4~{H}-thieno[3,2-c]chromene-2-carboxylic acid | C12 H8 O3 S | 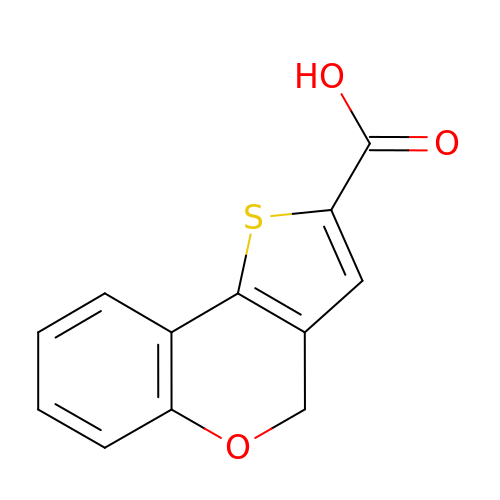ZMEWPWRPNHFDRC-UHFFFAOYSA-N>[3x]STLLASLRDWLKAQQLDAVLLSSRQNKQPHLGISTGSGYVVISRESAHILVDSRYYVEVEARAQGYQLHLLDATNTLTT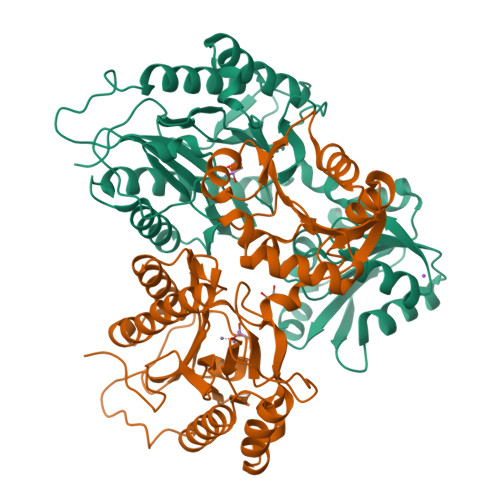IVNQIIADEQLQTLGFEGQQVSWETAHRWQSELNAKLVSATPDVLRQIKTPEEVEKIRLACGIADRGAEHIRRFIQAGMSEREIAAELEWFMRQQGAEKASFDTIVASGWRGALPHGKASDKIVAAGEFVTLDFGALYQGYCSDMTRTLLVNGEGVSAESHLLFNVYQIVLQAQLAAISAIRPGVRCQQVDDAARRVITEAGYGDYFGHNTGHAIGIEVHEDPRFSPRDTTTLQPGMLLTVEPGIYLPGQGGVRIEDVVLVTPQGAEVLYAMPKTVLLTGEA>HMFMAENRLQLQKGSAEETIERFYNRQGIETIEGFQQMFVTKTLNTEDTDEVKILTIWESEDSFNNWLNSDVFKEAHKNVRL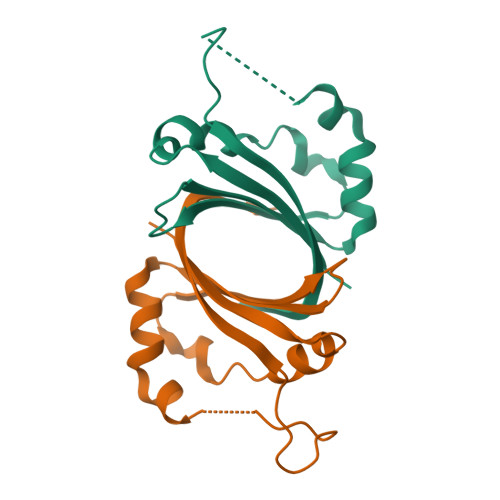KSDDDGQQSPILSNKVFKYDIGYHYQK[2x]> MELTPREKDKLLLFTAALVAERRLARGLKLNYPESVALISAFIMEGARDGKSVASLMEEGRHVLTREQVMEGVPEMIPDIQVEATFPDGSKLVTVHNPII;> MIPGEYHVKPGQIALNTGRATCRVVVENHGDRPIQVGSHYHFAEVNPALKFDRQQAAGYRLNIPAGTAVRFEPGQKREVELVAFAGHRAVFGFRGEVMGPLEVNDE;> MSNISRQAYADMFGPTVGDKVRLADTELWIEVEDDLTTYGEEVKFGGGKVIRDGMGQGQMLAADCVDLVLTNALIVDHWGIVKADIGVKDGRIFAIGKAGNPDIQPNVTIPIGAATEVIAAEGKIVTAGGIDTHIHWICPQQAEEALVSGVTTMVGGGTGPAAGTHATTCTPGPWYISRMLQAADSLPVNIGLLGKGNVSQPDALREQVAAGVIGLKIHEDWGATPAAIDCALTVADEMDIQVALHSDTLNESGFVEDTLAAIGGRTIHTFHTEGAGGGHAPDIITACAHPNILPSSTNPTLPYTLNTIDEHLDMLMVCAHLDPDIAEDVAFAESRIRRETIAAEDVLHDLGAFSLTSSDSQAMGRVGEVILRTWQVAHRMKVQRGALAEETGDNDNFRVKRYIAKYTIN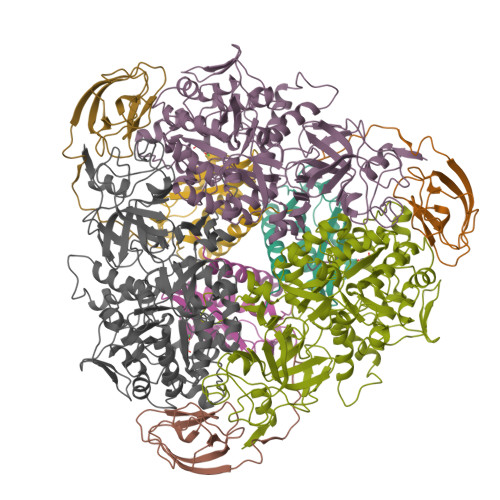PALTHGIAHEVGSIEVGKLADLVVWSPAFFGVKPATVIKGGMIAIAPMGDINASIPTPQPVHYRPMFGALGSARHHCRLTFLSQAAAANGVAERLNLRSAIAVVKGCRTVQKADMVHNSLQPNITVDAQTYEVRVDGELITSEPADVLPMAQRYFLF> APEYWCSIAYFEMDVQVGETFKVPSSCPIVTVDGYVDPSGGDRFCLGQLSNVHRTEAIERARLHIGKGVQLECKGEGDVWVRCLSDHAVFVQSYYLDREAGRAPGDAVHKIYPSAYIKVFDLRQCHRQMQQQAATAQAAAAAQAAAVAGNIPGPGSVGGIAPAISLSAAAGIGVDDLRRLCILRMSFVKGWGPDYPRQSIKETPCWIEIHLHRALQLLDE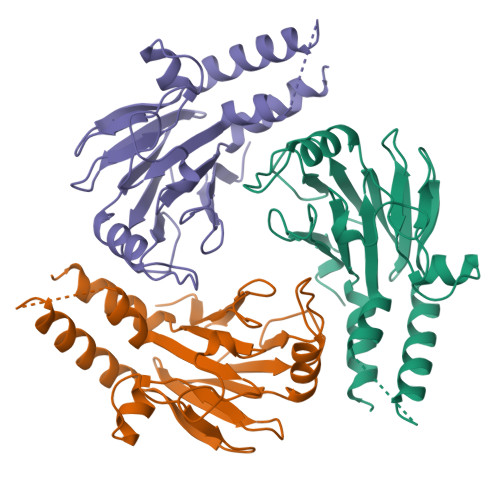VLHTMPIADPQPLD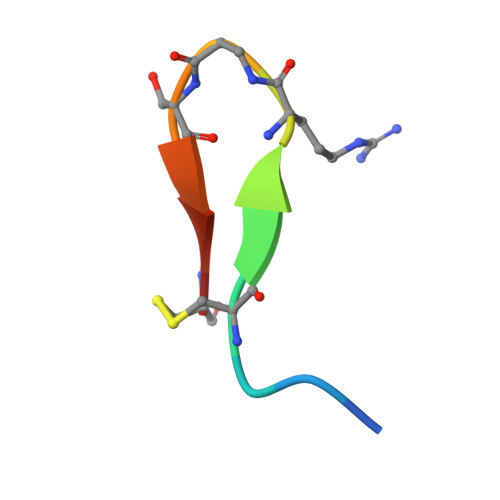> APYCVYRXSWSCX> DQYSLVASLDNVRNLSTILKAIHFREHATCFATKNGIKVTVENAKCVQANAFIQAGIFQEFKVQEESVTFRINLTVLLDCLSIFGSSPMPGTLTALRMCYQGYGYPLMLFLEEGGVVTVCKINTQEPEETLDFDFCSTNVINKIILQSEGLREAFSELDMTSEVLQITMSPD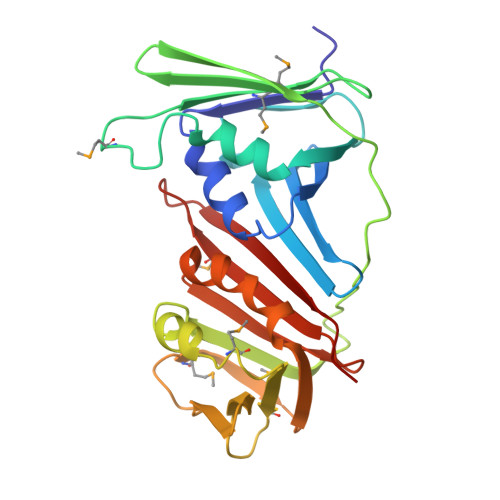KPYFRLSTFGNAGSSHLDYPKDSDLMEAFHCNQTQVNRYKISLLKPSTKALVLSCKVSIRTDNRGFLSLQYMIRNEDGQICFVEYYCCPDE>[2x]MGDLSCPEGLEELLSAPPPDLGAQRRHGWNPKDCSENIEVK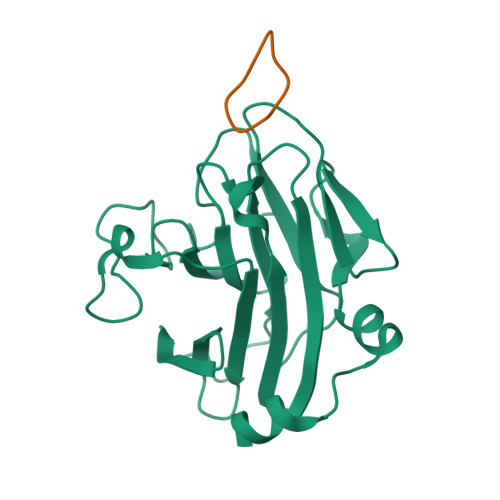EGGLYFERRPVAQSTDGARGKRGYSRGLHAWEISWPLEQRGTHAVVGVATALAPLQTDHYAALLGSNSESWGWDIGRGKLYHQSKGPGAPQYPAGTQGEQLEVPERLLVVLDMEEGTLGYAIGGTYLGPAFRGLKGRTLYPAVSAVWGQCQVRIRYLGERGSHHHHHH;>[2x]RGDINNNVE> MIKVEIKPSQAQFTTRSGVSRQGKPYSLNEQLCYVDLGNEYPVLVKVTLDEGQPA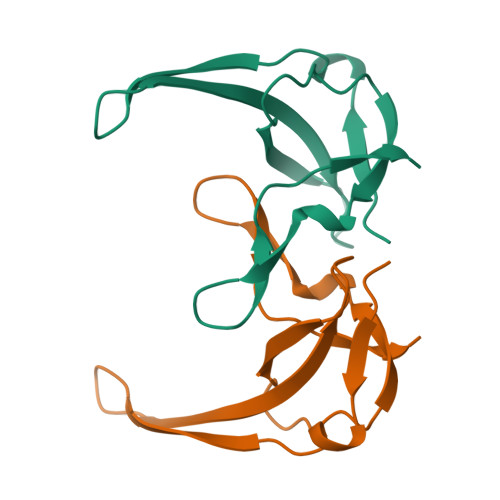YAPGLYTVHLSSFKVGQFGSLMIDRLRLVPAK>[2x]AHHHHHHMVHITLDRNTANSWLIISKDRRQVRMGDTHQ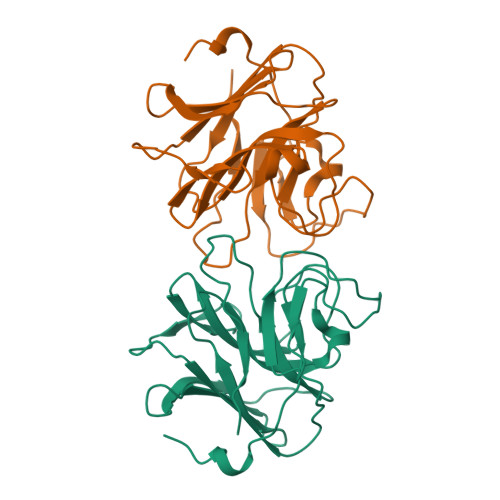NVSDNKERFSNYPMVLGAQRFSSGKMYWEVDVTQKEAWDLGVCRDSVQRKGQFSLSPENGFWTIWLWQDSYEAGTSPQTTLHIQVPPCQIGIFVDYEAGVVSFYNITDHGSLIYTFSECVFAGPLRPFFNVGFNYSGGNAAPLKLCPLKM>[4x]MSLANWYLDNESSRLSFTSTKNADIAE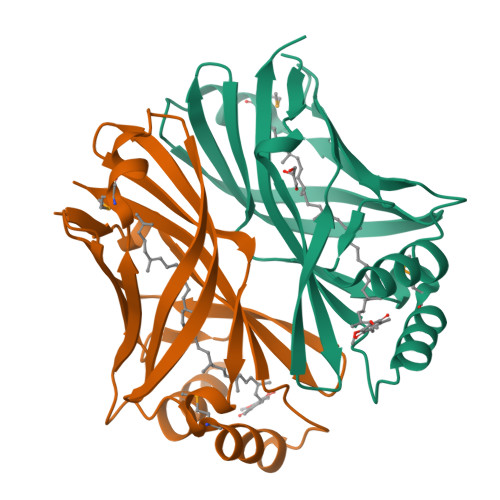VHRFLVLHGKVDPKGLAEVEVETESISTGIPLRDERLREQVFQVHKFPVAQINAQLDMRPINNLAPGAQLELRLPLTVSLRGKSHSYNAELLATRLDERRFQVVTLEPLVIHAQDFDMVSDFNALRNAAGLSAVSLSVPVGAVLIFTAREGHHHHHH> GNKICQFKLV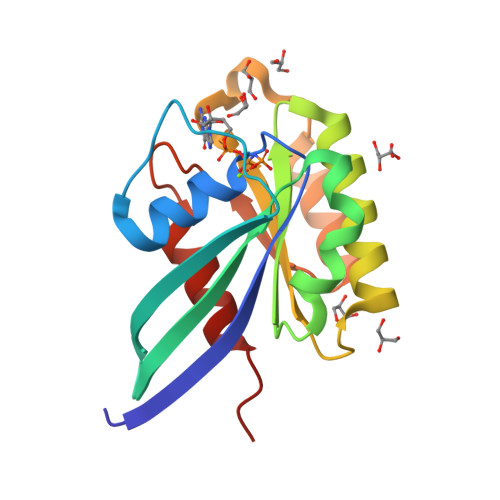LLGESAVGKSSLVLRFVKGQFHEFQESTIGAAFLTQTVCLDDTTVKFEIWDTAGQERYHSLAPMYYRGAQAAIVVYDITNEESFARAKNWVKELQRQASPNIVIALSGNKADLANKRAVDFQEAQSYADDNSLLFMETSAKTSMNVNEIFMAIAKKLPKN> MSRLDKSKVINSAL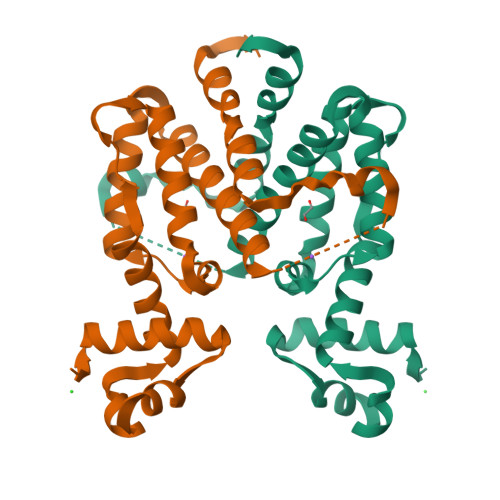ELLNEVGIEGLTTRKLAQKLGVEQPTLYWHVKNKRALLDALAVEILARHHDYSLPAAGESWQSFLRNNAMSFRRALLRYRDGAKVHLGTRPDEKQYDTVETQLRFMTENGFSLRDGLYAISWVSHFTLGAVLEQQEHTAALTDRPAAPDENLPPLLREALQIMDSDDGEQAFLHGLESAIRGIEVQLTALLQIV;> GSHMSRLDKSKVINSALELLNEVGIEGLTTRKLAQKLGVEQPTLYWHVKNKRALLDALAVEILARHHDYSLPAAGESWQSFLRNNAMSFRRALLRYRDGAKVHLGTRPDEKQYDTVETQLRFMTENGFSLRDGLYAISAVSHATLGAVLEQQEHTAALTDRPAAPDENLPPLLREALQIMDSDDGEQAFLHGLEWLIRGFEVQLTALLQIV> ACYIYQLPSWVLDDLCRNMDALSEWDWMEFASYVITDLTQLRKIKSMEWVQGVSITRELLWWWGMRQATVQQ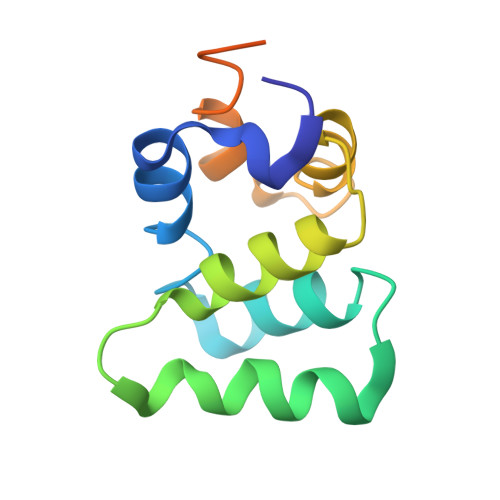LVDLLCRLELYRAAQIILNWKPAPEIRCPIPAFPDSVKP>[10x]GPGHMNSFVGLRVVAKWSSNGYFYSGKITR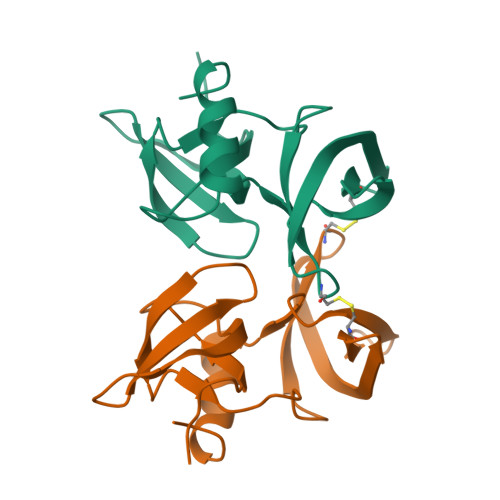DVGAGKYKLLFDDGYECDVLGKDILLCDPIPLDTEVTALSCDEYFSAGVVKGHRKESGCLYYSIEKEGQRKWYKRMAVILSLEQGNRLREQYGLG>[2x]SMKGSGQIQLWQFLLEL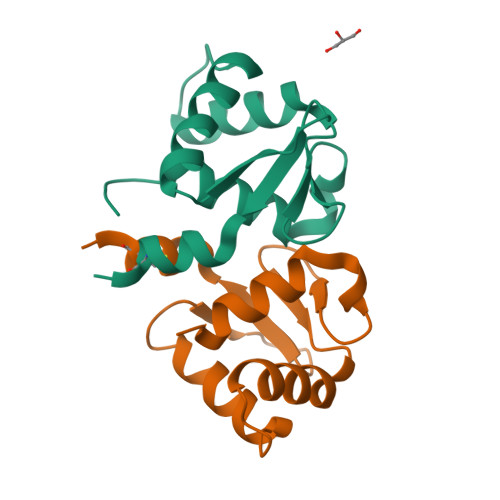LADRANAGCIAWEGGHGEFKLTDPDEVARRWGERKSKPNMNYDKLSRALRYYYDKNIMSKVHGKRYAYRFDFQGLAQACQPPPAH>KKMAFTLADRVTEEMLADKAALVVEVVEENYHDAPIVGIAVVNEHGRFFLRPETALADPQFVAWLGDETKKKSMFDSKRAAVALKWKGIELCGVSFDLLLAAYLLDPAQGV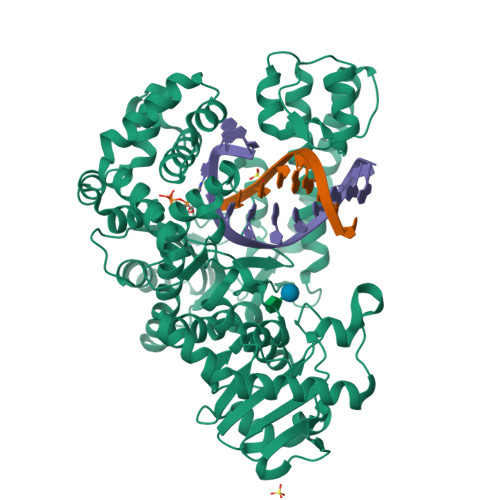DDVAAAAKMKQYEAVRPDEAVYGKGAKRAVPDEPVLAEHLVRKAAAIWELERPFLDELRRNEQDRLLVELEQPLSSILAEMEFAGVKVDTKRLEQMGKELAEQLGTVEQRIYELAGQEFNINSPKQLGVILFEKLQLPVLKKTKTGYSTSADVLEKLAPYHEIVENILHYRQLGKLQSTYIEGLLKVVRPATKKVHTIFNQALTQTGRLSSTEPNLQNIPIRLEEGRKIRQAFVPSESDWLIFAADYSQIELRVLAHIAEDDNLMEAFRRDLDIHTKTAMDIFQVSEDEVTPNMRRQAKAVNYGIVYGISDYGLAQNLNISRKEAAEFIERYFESFPGVKRYMENIVQEAKQKGYVTTLLHRRRYLPDITSRNFNVRSFAERMAMNTPIQGSAADIIKKAMIDLNARLKEERLQAHLLLQVHDELILEAPKEEMERLCRLVPEVMEQAVTLRVPLKVDYHYGSTWYDAK[2x]> MAKQYDSVECPFCDEVSKYEKLAKIGQGTFGEVFKARHRKTGQKVALKKVLMENEKEGFPITALREIKILQLLKHENVVNLIEICRTKASPYNRCKGSIYLVFDFCEHDLAGLLSNVLVKFTLSEIKRVMQMLLNGLYYIHRNKILHRDMKAANVLITRDGVLKLADFGLARAFSLAKNSQPNRYTNRVVTLWYRPPELLLGERDYGPPIDLWGAGCIMAEMWTRSPIMQGNTEQHQLALISQLCGSITPEVWPNVDNYELYEKLELVKGQKRKVKDRLKAYVRDPYALDLIDKLLVLDPAQRIDSDDALNHDFFWSDPMPSDLKGMLST;> MEGERKNNNKRWYFTREQLENSPSRRFGVDPDKELSYRQQAANLLQDMGQRLNVSQLTINTAIVYMHRFYMIQSFTQFPGNSVAPAALFLAAKVEEQPKKLEHVIKVAHTCLHPQESLPDTRSEAYLQQVQDLVILESIILQTLGFELTIDHPHTHVVKCTQLVRASKDLAQTSYFMATNSLHLTTFSLQYTPPVVACVCIHLACKWSNWEIPVSTDGKHWWEYVDATVTLELLDELTHEFLQILEKTPNRLKRIWNWRACEAA;> SPLFAEPYKVTSKEDKLSSRIQSMLGNYDEMKDFIG;> XMEPVDPRLEPWKHPGSQPKTACTNCYCKKCCFHCQVCFITKALGISYG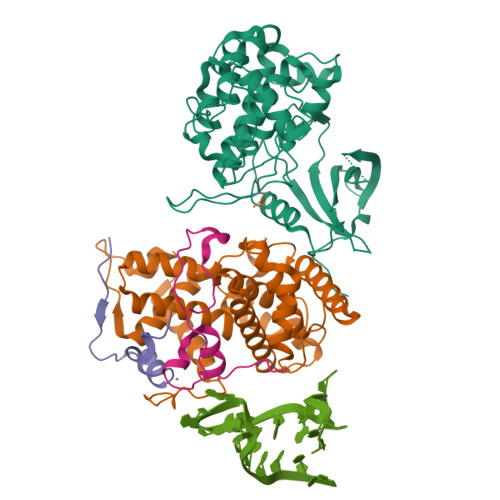RKKRRQRRR> KTSGKGKLPPVYPVTVPFLGHIVQFGKNPLEFMQRCKRDLKSGVFTISIGGQRVTIVGDPHEHSRFFSPRNEILSPREVYTIMTPVFGEGVAYAAPYPRMREQLNFLAEELTIAKFQNFVPAIQHEVRKFMAENWKEDEGVINLLEDCGAMIINTACQCLFGEDLRKRLNARHFAQLLSKMESSLIPAAVFMPWLLRLPLPQSARCREARAELQKILGEIIVAREKEEASKDNNTSDLLGGLLKAVYRDGTRMSLH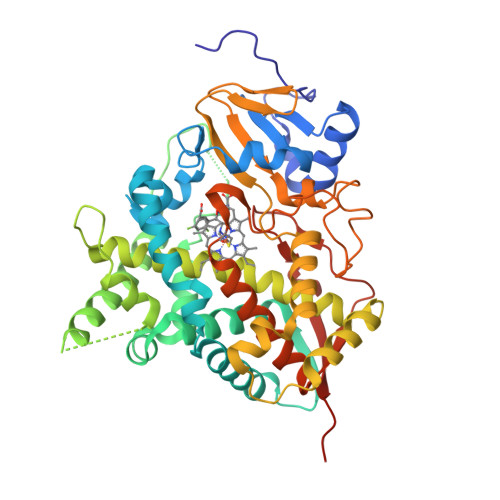EVCGMIVAAMFAGQHTSTITTSWSMLHLMHPKNKKWLDKLHKEIDEFPAQLNYDNVMDEMPFAERCVRESIRRDPPLLMVMRMVKAEVKVGSYVVPKGDIIACSPLLSHHDEEAFPNPRLWDPERDEKVDGAFIGFGAGVHKCIGQKFALLQVKTILATAFREYDFQLLRDEVPDPDYHTMVVGPTLNQCLVKYTRKKKLPSHHHHHH> GSAMGSASTSGNP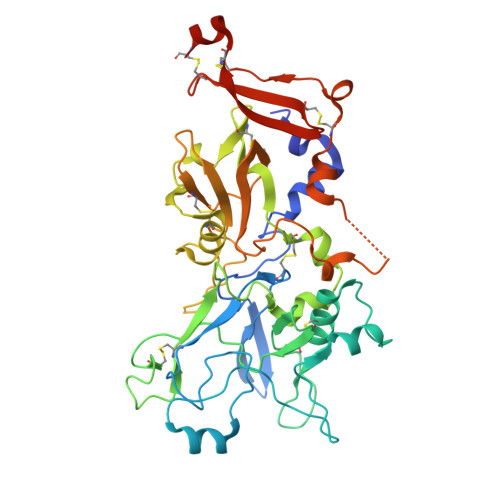FQANVEMKTFMERFNLTHHHQSGIYVDLGQDKEVDGTLYREPAGLCPIWGKHIELQQPDRPPYRNNFLEDVPTEKEYKQSGNPLPGGFNLNFVTPSGQRISPFPMELLEKNSNIKASTDLGRCAEFAFKTVAMDKNNKATKYRYPFVYDSKKRLCHILYVSMQLMEGKKYCSVKGEPPDLTWYCFKPRKSVTENHHLIYGSAYVGENPDAFISKCPNQALRGYRFGVWKKGRCLDYTELTDTVIERVESKAQCWVKTFENDGVASDQPHTYPLTSQASWNDWWPLHQSDQPHSGGVGRNYGFYYVDTTGEGKCALSDQVPDCLVSDSAAVSYTAAGSLSEETPNFIIPSNPSVTPPTPETALQCTADKFPDSFGACDVQACKRQKTSCVGGQIQSTSVDCTADEQNECGSNTAAALVPR> MGNDQPHVVVCSGAGMGHLTPFLNLASALSSAPYNCKVTLLIVIPLITDAESHHISSFFSSHPTIHRLDFHVNLPAPKPNVDPFFLRYKSISDSAHRLPVHLSALSPPISAVFSDFLFTQGLNTTLPHLPNYTFTTTSARFFTLMSYVPHLAKSSSSSPVEIPGLEPFPTDNIPPPFFNPEHIFTSFTISNAKYFSLSKGILVNTFDSFEPETLSALNSGDTLSDLPPVIPIGPLNELEHNKQEELLPWLDQQPEKSVLYVSFGNRTAMSSDQILELGMGLERSDCRFIWVVKTSKIDKDDKSELRKLFGEELYLKLSEKGKLVKWVNQTEILGHTAVGGFLSHCGWNSVMEAARRGVPIL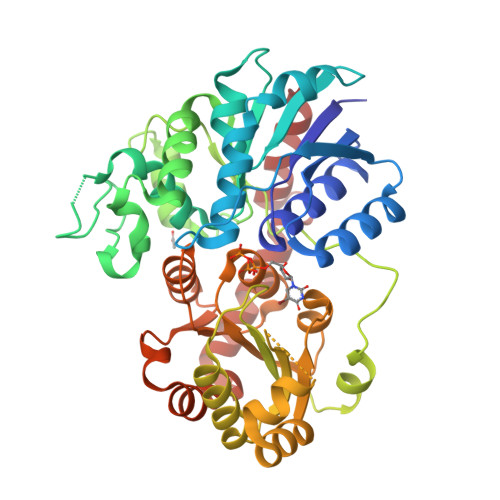AWPQHGDQRENAWVVEKAGLGVWEREWASGIQAAIVEKVKMIMGNNDLRKSAMKVGEEAKRACDVGGSSATALMNIIGSLKR>MSDKPIDIQYDKQATPNLSGVITPPTNETGNDSVREKLSKLVGDAMSNNPYFAAGGGLMILGTGLAVARSGIIKASRVLYRQMIVDLEIQSKDKSYAWFLTWMAKHPQRVSRHLSVRTNYIQHDNGSVSTKFSLVPGPGNHWIRYKGAFILIKRERSAKMIDIANGSPFETVTLTTLYRDKHLFDDILNEAKDIALKTTEGKTVIYTSFGPEWRKFGQPKAKRMLPSVILDSGIKEGILDDVYDFMKNGKWYSDRGIPYRRGYLLYGPPGSGKTSFIQALAGELDYNICILNLSENNLTDDRLNHLMNNMPERSILLL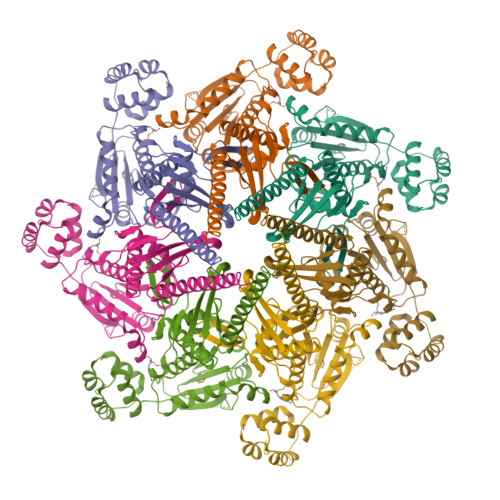EDIDAAFNKRSQTGEQGFHSSVTFSGLLNALDGVTSSEETITFMTTNHPEKLDAAIMRPGRIDYKVFVGNATPYQVEKMFMKFYPGETDICKKFVNSVKELDITVSTAQLQGLFVMNKDAPHDALKMVSSLRNANHIF[7x]>GPGSEFLDGDLDPGLPSTEDVILKTEQVTKNIQELLRAAQEFKHDSFVPCSEKIHLAVTEMASLFPKRPALEPVRSSLRLLNASAYRLQSECRKTVPPEPGAPVDFQLLTQQVIQCAYDIAKAAKQLVTITTREKKQ[2x];>[2x]GSGSGSGSGSSATRELDELMASLSDFKM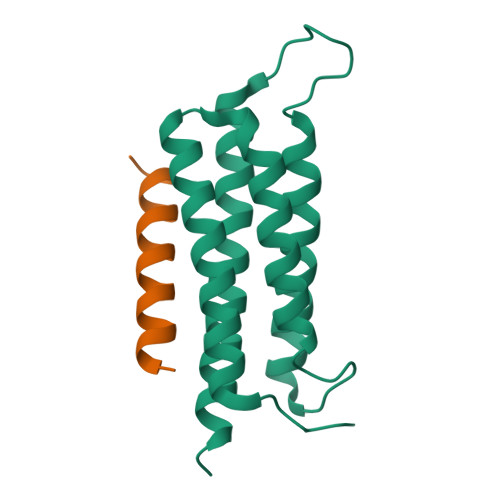QGLE ICV, however, has only one major surface glycoprotein, the hemagglutinin-esterase-fusion (HEF) protein, which possesses all-in-one of receptor binding, receptor destroying and membrane fusion activities. To further evaluate the infectivity and transmissibility of IDV, we expressed and purified the ectodomain of D/OK HEF, and determined that it also uses 9-O-Acetyl-Sia as its receptor by glycan microarray. We also solved the crystal structure of D/OK HEF, both in its native state (resolution of 2.4 Å) and in complex with its receptor analogue (resolution of 3.1 Å), and the structure of the enzymatically inactive HEF (resolution of 2.4 Å) alone and in complex with two receptor analogs respectively (both resolutions of 2.2 Å). Indeed, our results show that IDV HEF is functionally and structurally similar to ICV HEF, but with some distinct characteristics.

To avoid the enzymatic cleavage of the receptor substrates, we generated the catalytic mutant for the binding experiments and for the structures of the relevant complexes. Previous studies have demonstrated that the residues S57, D356 and H359 create a catalytic triad in ICV HEF esterase, which has been proved by site-directed mutagenesis and structural analysis, and the sequence alignment between the ICV and IDV HEF proteins reveals that a highly conserved catalytic triad is also observed in IDV HEF protein. Thus, we designed the enzymatically inactive HEF protein (HEF-mut) containing S57A, D356A and H359A substitutions, and expressed it using the same method as wild type protein. In order to study the molecular basis of IDV HEF and its receptor / substrate binding mode we solved the native X-ray crystallography structures of wild type and mutant HEFs both at a resolution of 2.4 Å. Secondly, we performed an enzyme kinetics assay using pNPA as a substrate at three different temperatures (37°C, 25°C and 4°C). Both IDV and ICV HEF displayed obvious esterase activities while HEF-mut proteins exhibited no enzymatic activities. Due to the presence of cacodylate buffer in the crystallization conditions, S57 in our IDV HEF structure is covalently modified by the addition of a dimethylarsenic group.

>ELICIVQRVNESFSLHSGFGGNVYSMKTEPMTGFTNVTKGASVINQKDWIGFGDARTDLTNDQFPASSDVPLAVAKKFRSLSGASLMLSAFGPPGKVDYLYQGCGKEKVFYEGVNWSPEAGIDCFGSNWTQTKKDFYSRIYEAARSSTCMTLVNSLDTKISSTTATAGTASSCSSSWMKSPLWYAESSVNPGAKPQVCGTEQSATFTLPTSFGIYKCNKHVVQLCYFVYENKAKFNTFGCGDYYQNYYDGNGNLIGGMDNRVAAYRGIANAGVKIECPSKILNPGTYSIKSTPRFLLVPKRSYCFDTDGGYPIQVVQSEWSASRRSDNATEEACLQTEGCIFIKKTTPYVGEAADNAGDIEMRQLLSGLGNNDTVCVSQSGYTKGETPFVKDYLSPPKYGRCQLKTDSGRIPTLPSGLIIPQAGTDS[2x];>IFGIDDLIFGLLFVGFVAGGVAGGYFWGRSNGGGGGASVSSTQAGFDKIGKDIQQLRNDTNAAIEGFNGRIAHDEQAIKNLAKEIEDARAEALVGELGIIRSLIVANISMNLKESLYELANQITKRGGGIAQEAGPGCWYVDSENCDASCKEYIFNF[2x]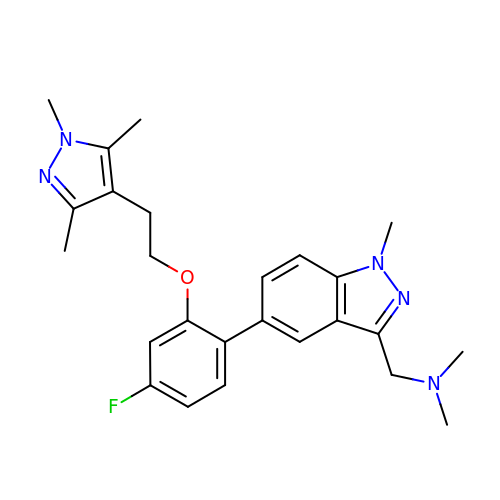1-(5-{4-fluoro-2-[2-(1,3,5-trimethyl-1H-pyrazol-4-yl)ethoxy]phenyl}-1-methyl-1H-indazol-3-yl)-N,N-dimethylmethanamine | C25 H30 F N5 O | YEOAAQMCKFJWKF-UHFFFAOYSA-N>[4x]YSINNSRQIVDDSGKVVQLKGVNVFGFETGNHVMHGLWARNWKDMIVQMQGLGFNAVRLPFCPATLRSDTMPASIDYSRNADLQGLTSLQILDKVIAEFNARGMYVLLDHHTPDCAGISELWYTGSYTEAQWLADLRFVANRYKNVPYVLGLDLKNEPHGAATWGTGNAATDWNKAAERGSAAVLAVAPKWLIAVEGITDNPVCSTNGGIFW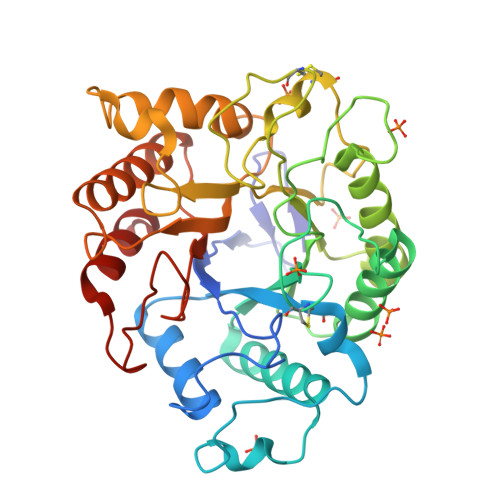GGNLQPLACTPLNIPANRLLLAPHVYGPDVFVQSYFNDSNFPNNMPAIWERHFGQFAGTHALLLGEFGGKYGEGDARDKTWQDALVKYLRSKGINQGFYWSWNPNSGDTGGILRDDWTSVRQDKMTLLRTLWGT>KHPLRVGVGGPVGSGKTALLEALCKAMRDTWQLAVVTNDIYTKEDQRILTEAGTLAPERIVGVETGGCPHTAIREDASMNLAAVEALSEKFGNLDLIFVESGGDNLSATFSPELADLTIYVIDVAEGEKI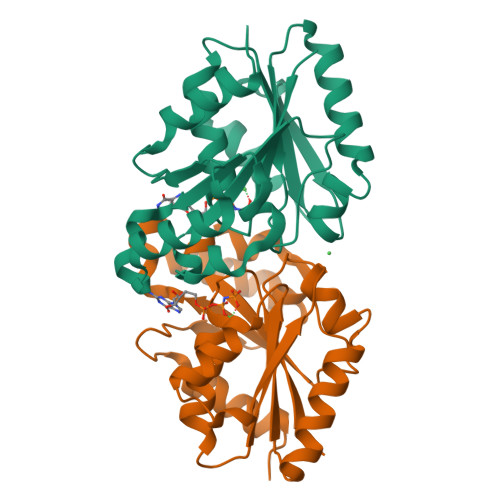PRKGGPGITRSDFLVINKTDLAPYVGASLKVMASDTQRMRGDRPWTFTNLKQGDGLSTIIAFLEDKGMLG[2x]> QEITVDEFSNIRENPVTPWNPEPSAPVIDPTAYIDPQASVIGEVTIGANVMVSPMASIRSDEGMPIFVGDRSNVQDGVVLHALETINEEGEPIEDNIVEVDGKEYAVYIGNNVSLAHQSQVHGPAAVGDDTFIGMQAFVF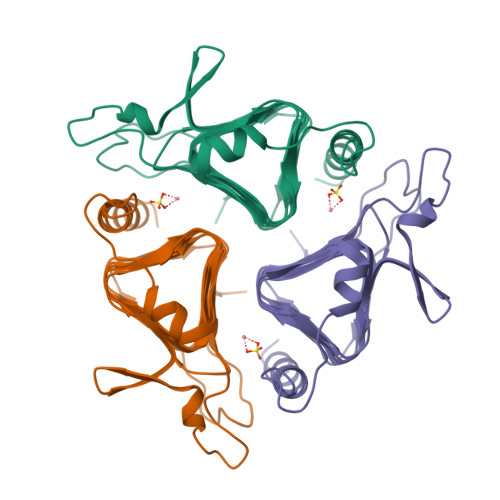KSKVGNNCVLEPRSAAIGVTIPDGRYIPAGMVVTSQAEADKLPEVTDDYAYSHTNEAVVYVNVHLAEGYKETS>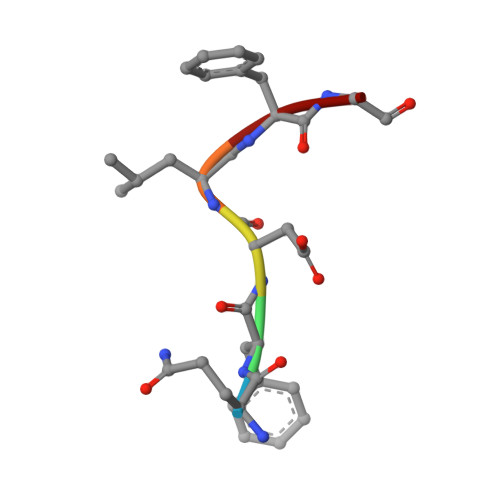 QFDLFG>MRLTILGMTAHDSRPEQAKKLADIDWSTLGFSYIRTDLRYLAHWKDGEWDAGTLTEDNQIHLAEGSTALHYGQQCFEGLKAYRCADGSINLFRPDQNAARMRMSCRRLLMPELSDEQFIDACLQVVRANEHFLPPYGTGGSLYLRPFVIGVGDNIGVRTAPEFIFSVFCVPVGPYFKGGLTPTNFITSDYDRAAPHGTGAAKVGGNYAASLLPGYEAKKRDFADVIYLDPATHTTIEEAGAANFFAITQDGQKFVTPQSPSILPSITKYSLLWLAEHRLGLEVEEGDIRIDELGKFSEAGACGTAAVITPIGGIQHGDDFHVFYSESEPGPVTRRLYDELVGIQYGDKEAPE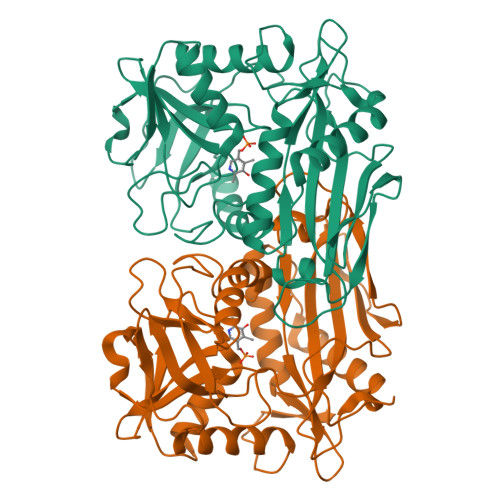GWIVKV[2x]> GPSQDASDGLQRLHMLQISYFRDPYHVWYQGNASLGGHLTHVLEGPDTNTTIIQLQPLQEPESWARTQSGLQSYLLQFHGLVRLVHQERTLAFPLTIRCFLG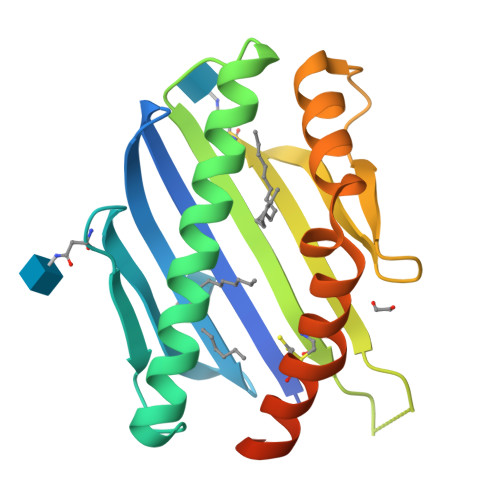CELPPEGSRAHVFFEVAVNGSSFVSFRPERALWQADTQVTSGVVTFTLQQLNAYNRTRYELREFLEDTCVQYVQKHISAENTKGSQTSRSYTS N-(2-cyclohexylethyl)-3,5-dimethyl-1,2-oxazole-4-carboxamide 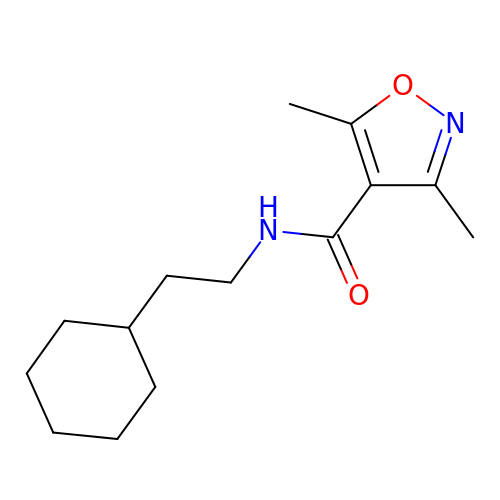| C14 H22 N2 O2 | GQYKDIBHTYIVTB-UHFFFAOYSA-N>ATRLTKKQLAQAIQNTLPNPPRRKRRAKRRAAQVPKPTQAGVSMAPIAQGTMVKLRPPMLRSSMDVTILSHCELSTELAVTVTIVVTSELVMPFTVGTWLRGVAQNWSKYAWVAIRYTYLPSCPTTTSGAIHMGFQYDMADTLPVSVNQLSNLKGYVTGPVWEGQSGLCFVNNTKCPDTSRAITIALDTNEVSEKRYPFKTATDYATAVGVNANIGNILV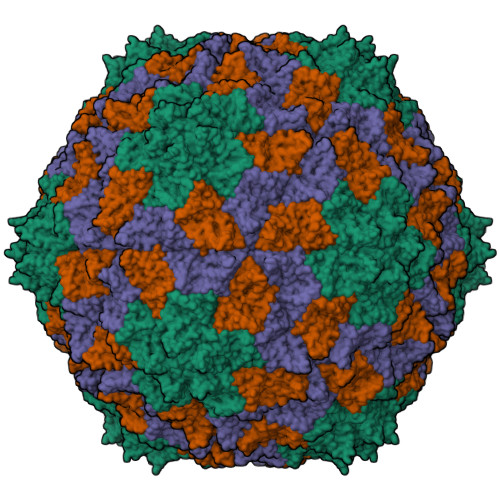PARLVTAMEGGSSKTAVNTGRLYASYTIRLIEPIAAALNL[3x]2-BROMO-2-CHLORO-1,1,1-TRIFLUOROETHANE | C2 H Br Cl F3 | 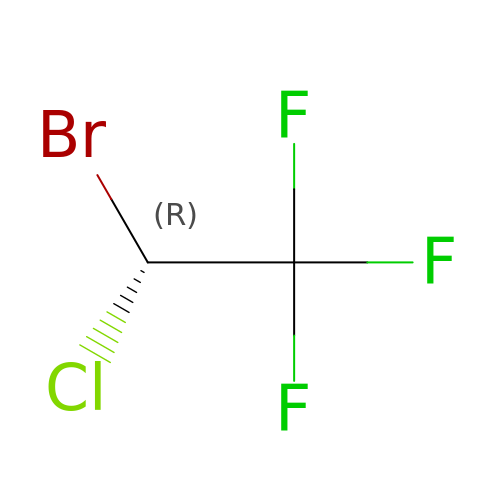BCQZXOMGPXTTIC-SFOWXEAESA-N>[6x]MTEKEKMLAEKWYDANFDQTLINERLRAKVICFALNHTNPVATMMRKVLIDALFQTTTDNVSISIPFDTDYGWNVKLGKNVYVNTNCYFMDGGQITIGDNVFIGPNCGFYTATH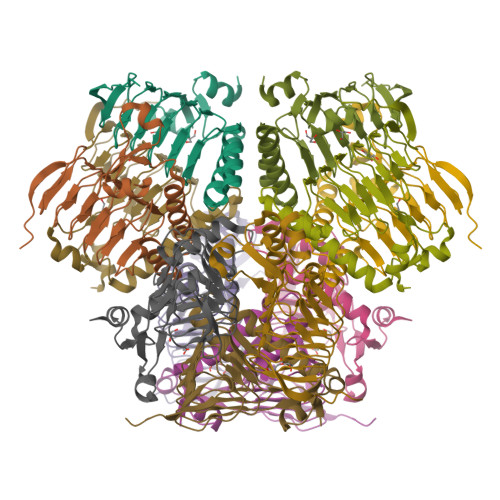PLNFHHRNEGFEKAGPIHIGSNTWFGGHVAVLPGVTIGEGSVIGAGSVVTKDIPPHSLAVGNPCKVVRKIDNDLPSETLNDETIKLEHHHHHH>[3x]MKPEVEQELAHILLTELLAYQFASPVRWIETQDVFLKDFNTERVVEIGPSPTLAGMAQRTLKNKYESYDAALSLHREILCYSKDAKEIYYTPDPSELAAKEEPAKEEAPAPTPAASAPAPAAAAPAPVAAAAPAAAAAEIADEPVKASLLLHVLVAHKLKKSLDSIPMSKTIKDLVGGKSTVQNEILGDLGKEFGTTPEKPEETPLEELAETFQDTFSGALGKQSSSLLSRLISSKMPGGFTITVARKYLQTRWGLPSGRQDGVLLVALSNEPAARLGSEADAKAFLDSMAQKYASIVGVDLSSAASASGAAGAGAAAGAAMIDAGALEEITKDHKVLARQQLQVLARYLKMDLDNGERKFLKEKDTVAELQAQLDYLNAELGEFFVNGVATSFSRKKARTFDSSWNWAKQSLLSLYFEIIHGVLKNVDREVVSEAINIMNRSNDALIKFMEYHISNTDETKGENYQLVKTLGEQLIENCKQVLDVDPVYKDVAKPTGPKTAIDKNGNITYSEEPREKVRKLSQYVQEMALGGPITKESQPTIEEDLTRVYKAISAQADKQDISSSTRVEFEKLYSDLMKFLESSKEIDPSQTTQLAGMDVEDALDKDSTKEVASLPNKSTISKTVSSTIPRETIPFLHLRKKTPAGDWKYDRQLSSLFLDGLEKAAFNGVTFKDKYVLITGAGKGSIGAEVLQGLLQGGAKVVVTTSRFSKQVTDYYQSIYAKYGAKGSTLIVVPFNQGSKQDVEALIEFIYDTEKNGGLGWDLDAIIPFAAIPEQGIELEHIDSKSEFAHRIMLTNILRMMGCVKKQKSARGIETRPAQVILPMSPNHGTFGGDGMYSESKLSLETLFNRWHSESWANQLTVCGAIIGWTRGTGLMSANNIIAEGIEKMGVRTFSQKEMAFNLLGLLTPEVVELCQKSPVMADLNGGLQFVPELKEFTAKLRKELVETSEVRKAVSIETALEHKVVNGNSADAAYAQVEIQPRANIQLDFPELKPYKQVKQIAPAELEGLLDLERVIVVTGFAEVGPWGSARTRWEMEAFGEFSLEGCVEMAWIMGFISYHNGNLKGRPYTGWVDSKTKEPVDDKDVKAKYETSILEHSGIRLIEPELFNGYNPEKKEMIQEVIVEEDLEPFEASKETAEQFKHQHGDKVDIFEIPETGEYSVKLLKGATLYIPKALRFDRLVAGQIPTGWNAKTYGISDDIISQVDPITLFVLVSVVEAFIASGITDPYEMYKYVHVSEVGNCSGSGMGGVSALRGMFKDRFKDEPVQNDILQESFINTMSAWVNMLLISSSGPIKTPVGACATSVESVDIGVETILSGKARICIVGGYDDFQEEGSFEFGNMKATSNTLEEFEHGRTPAEMSRPATTTRNGFMEAQGAGIQIIMQADLALKMGVPIYGIVAMAATATDKIGRSVPAPGKGILTTAREHHSSVKYASPNLNMKYRKRQLVTREAQIKDWVENELEALKLEAEEIPSEDQNEFLLERTREIHNEAESQLRAAQQQWGNDFYKRDPRIAPLRGALATYGLTIDDLGVASFHGTSTKANDKNESATINEMMKHLGRSEGNPVIGVFQ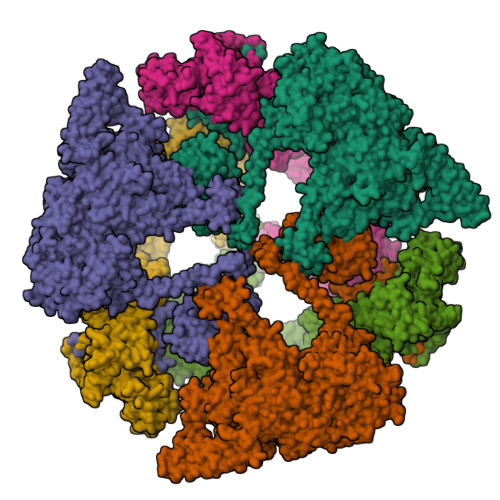KFLTGHPKGAAGAWMMNGALQILNSGIIPGNRNADNVDKILEQFEYVLYPSKTLKTDGVRAVSITSFGFGQKGGQAIVVHPDYLYGAITEDRYNEYVAKVSAREKSAYKFFHNGMIYNKLFVSKEHAPYTDELEEDVYLDPLARVSKDKKSGSLTFNSKNIQSKDSYINANTIETAKMIENMTKEKVSNGGVGVDVELITSINVENDTFIERNFTPQEIEYCSAQPSVQSSFAGTWSAKEAVFKSLGVKSLGGGAALKDIEIVRVNKNAPAVELHGNAKKAAEEAGVTDVKVSISHDDLQAVAVAVSTKK;>[3x]MDAYSTRPLTLSHGSLEHVLLVPTASFFIASQLQEQFNKILPEPTEGFAADDEPTTPAELVGKFLGYVSSLVEPSKVGQFDQVLNLCLTEFENCYLEGNDIHALAAKLLQENDTTLVKTKELIKNYITARIMAKRPFDKKSNSALFRAVGEGNAQLVAIFGGQGNTDDYFEELRDLYQTYHVLVGDLIKFSAETLSELIRTTLDAEKVFTQGLNILEWLENPSNTPDKDYLLSIPISCPLIGVIQLAHYVVTAKLLGFTPGELRSYLKGATGHSQGLVTAVAIAETDSWESFFVSVRKAITVLFFIGVRCYEAYPNTSLPPSILEDSLENNEGVPSPMLSISNLTQEQVQDYVNKTNSHLPAGKQVEISLVNGAKNLVVSGPPQSLYGLNLTLRKAKAPSGLDQSRIPFSERKLKFSNRFLPVASPFHSHLLVPASDLINKDLVKNNVSFNAKDIQIPVYDTFDGSDLRVLSGSISERIVDCIIRLPVKWETTTQFKATHILDFGPGGASGLGVLTHRNKDGTGVRVIVAGTLDINPDDDYGFKQEIFDVTSNGLKKNPNWLEEYHPKLIKNKSGKIFVETKFSKLIGRPPLLVPGMTPCTVSPDFVAATTNAGYTIELAGGGYFSAAGMTAAIDSVVSQIEKGSTFGINLIYVNPFMLQWGIPLIKELRSKGYPIQFLTIGAGVPSLEVASEYIETLGLKYLGLKPGSIDAISQVINIAKAHPNFPIALQWTGGRGGGHHSFEDAHTPMLQMYSKIRRHPNIMLIFGSGFGSADDTYPYLTGEWSTKFDYPPMPFDGFLFGSRVMIAKEVKTSPDAKKCIAACTGVPDDKWEQTYKKPTGGIVTVRSEMGEPIHKIATRGVMLWKEFDETIFNLPKNKLVPTLEAKRDYIISRLNADFQKPWFATVNGQARDLATMTYEEVAKRLVELMFIRSTNSWFDVTWRTFTGDFLRRVEERFTKSKTLSLIQSYSLLDKPDEAIEKVFNAYPAAREQFLNAQDIDHFLSMCQNPMQKPVPFVPVLDRRFEIFFKKDSLWQSEHLEAVVDQDVQRTCILHGPVAAQFTKVIDEPIKSIMDGIHDGHIKKLLHQYYGDDESKIPAVEYFGGESPVDVQSQVDSSSVSEDSAVFKATSSTDEESWFKALAGSEINWRHASFLCSFITQDKMFVSNPIRKVFKPSQGMVVEISNGNTSSKTVVTLSEPVQGELKPTVILKLLKENIIQMEMIENRTMDGKPVSLPLLYNFNPDNGFAPISEVMEDRNQRIKEMYWKLWIDEPFNLDFDPRDVIKGKDFEITAKEVYDFTHAVGNNCEDFVSRPDRTMLAPMDFAIVVGWRAIIKAIFPNTVDGDLLKLVHLSNGYKMIPGAKPLQVGDVVSTTAVIESVVNQPTGKIVDVVGTLSRNGKPVMEVTSSFFYRGNYTDFENTFQKTVEPVYQMHIKTSKDIAVLRSKEWFQLDDEDFDLLNKTLTFETETEVTFKNANIFSSVKCFGPIKVELPTKETVEIGIVDYEAGASHGNPVVDFLKRNGSTLEQKVNLENPIPIAVLDSYTPSTNEPYARVSGDLNPIHVSRHFASYANLPGTITHGMFSSASVRALIENWAADSVSSRVRGYTCQFVDMVLPNTALKTSIQHVGMINGRKLIKFETRNEDDVVVLTGEAEIEQPVTTFVFTGQGSQEQGMGMDLYKTSKAAQDVWNRADNHFKDTYGFSILDIVINNPVNLTIHFGGEKGKRIRENYSAMIFETIVDGKLKTEKIFKEINEHSTSYTFRSEKGLLSATQFTQPALTLMEKAAFEDLKSKGLIPADATFAGHSLGEYAALASLADVMSIESLVEVVFYRGMTMQVAVPRDELGRSNYGMIAINPGRVAASFSQEALQYVVERVGKRTGWLVEIVNYNVENQQYVAAGDLRALDTVTNVLNFIKLQKIDIIELQKSLSLEEVEGHLFEIIDEASKKSAVKPRPLKLERGFACIPLVGISVPFHSTYLMNGVKPFKSFLKKNIIKENVKVARLAGKYIPNLTAKPFQVTKEYFQDVYDLTGSEPIKEIIDNWEKYEQS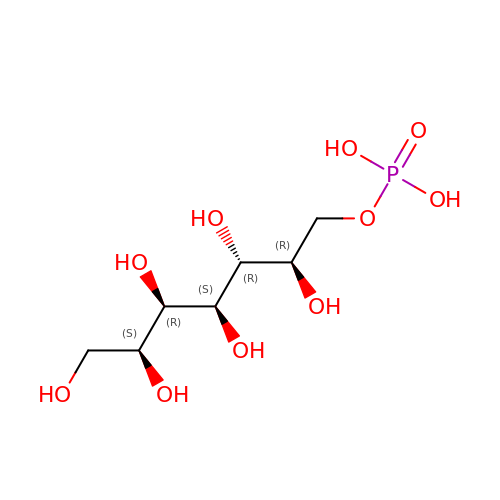(2R,3R,4S,5R,6S)-2,3,4,5,6,7-hexahydroxyheptyl dihydrogen phosphate | C7 H17 O10 P | RCCDYOCQCITNBH-CJZRUXIPSA-N> MSSEHRCIDTNVPENAACYRYLDGTEEWRCLLYFKEDAGKCVPAPNMTCKDKNGGCAPEAECK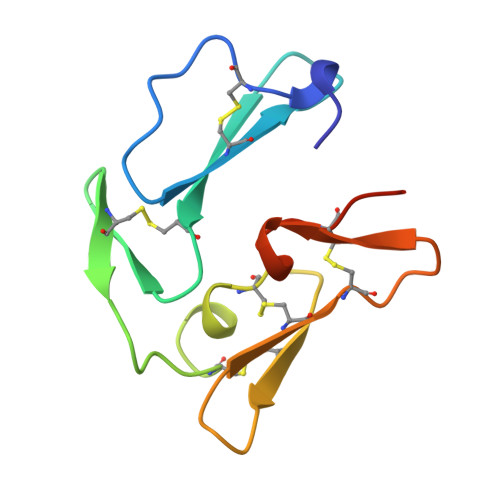MNDKNEIVCKCTKEGSEPLFEGVFCSHHHHHH>[2x]VKQVFNFNAGPSALP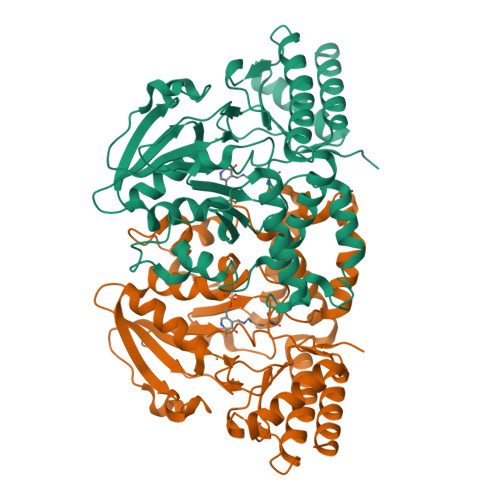KPALERAQKELLNFNDTQMSVMELSHRSQSYEEVHEQAQNLLRELLQIPNDYQILFLQGGASLQFTMLPMNLLTKGTIGNYVLTGSWSEKALKEAKLLGETHIAASTKANSYQSIPDFSEFQLNENDAYLHITSNNTIYGTQYQNFPEINHAPLIADMSSDILSRPLKVNQFGMIYAGAQKNLGPSGVTVVIVKKDLLNTKVEQVPTMLQYATHIKSDSLYNTPPTFSIYMLRNVLDWIKDLGGAEAIAKQNEEKAKIIYDTIDESNGFYVGHAEKGSRSLMNVTFNLRNEELNQQFLAKAKEQGFVGLNGHRSVGGCRASIYNAVPIDACIALRELMIQFKENA>SDKIIHLTDDSFDTDVLKADGAILVDFWAEWCGPCKMIAPILDEIADEYQGKLTVAKLNIDQNPGTAPKYGIRGIPTLLLFKNGEVAATKVGAL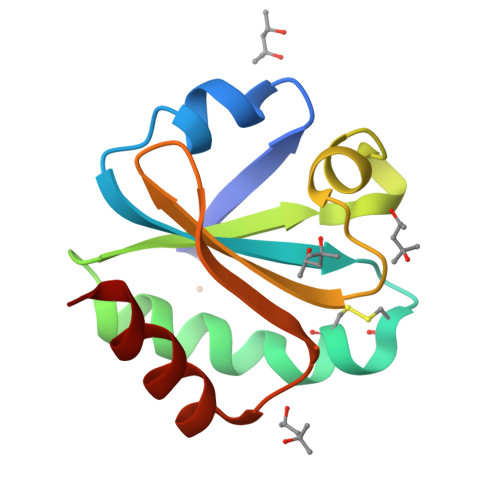SKGQLKEFLDANLA[2x]> MWLGALLDTLPTPALTIDRTTARRNAERMRERCRALGVRLRPHVKTHKTLEGGLLATGGTRRGIAVSTLAEARFFADGGFDD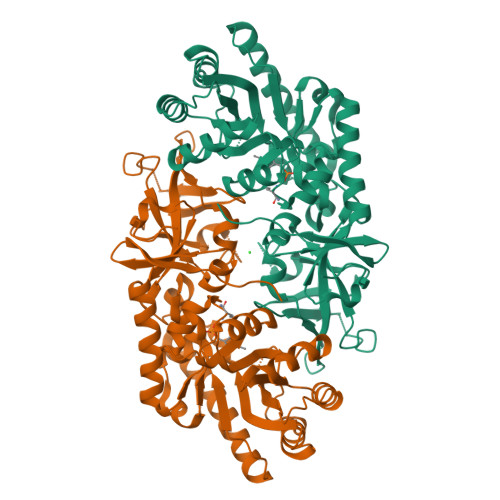ILLAYPVPTARLEECAGLARRLDAFHVLLDRPEALASLRQRPLGHGKRWLVWLKLDCGNGRAGVRPTDPAALELAQAIANDAPEEVTLVGVYAHCGNTYGCSGADTIQAIARTTTNAVLSFVAALRQAGVPCPQASIGSTPSCSHPIPEMSQLTELHPGNYIFYDLQQTQLGSCQPQDVAIRVLTRVIGHYAHRGQLLVDCGWAALSLHGAGAGQGPQGCAAIDGHPELRLVGLTQEHGLLEHAGGQMDFGRFPVGSVLALIPYHACATAAMHPVYYVHEEGKVVALWHPVRGW> SNAMATDFSKLSKYVETLRVKPKQSIDLKKDFDTDYDHKMLTKEEGEELLNLGISKLSEIQEKLYASGTKSVLIVFQAMDAAGKDGTVKHIMTGLNPQGVKVTSFKVPSKIELSHDYLWRHYVALPATGEIGIFNRSHYENVLVTRVHPEYLLSEQTSGVTAIEQVNQKFWDKRFQQINNFEQHISENGTIVLKFFLHVSKKEQKKRFIERIELDTKNWKFSTGDLKERAHWKDYRNAYEDMLANTSTKQAPWFVIPADDKWFTRLLIAEIICTELEKLNLTFPTVSLEQKAELEKAK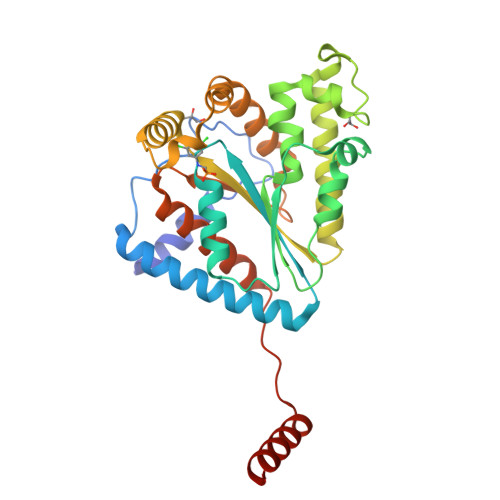AELVAEKSSD> GSHMLSDEQMQIINSLVEAHHKTYDDSYSDFVRFRPPVREGPVTRSASRAASLHSLSDASSDSFNHSPESVDTKLNFSNLLMMYQDSGSPDSSEEDQQSRLSMLPHLADLVSYSIQKVIGFAKMIPGFRDLTAEDQIALLKSSAIEIIMLRSNQSFSLEDMSWSCGGPDFKYCINDVTKAGHTLEHLEPLVKFQVGLKKLKLHEEEHVLLMAICLLSPDRPGVQDHVRIEALQDRLCDVLQAYIRIQHPGGRLLYAKMIQKLADLRSLNEEHSKQY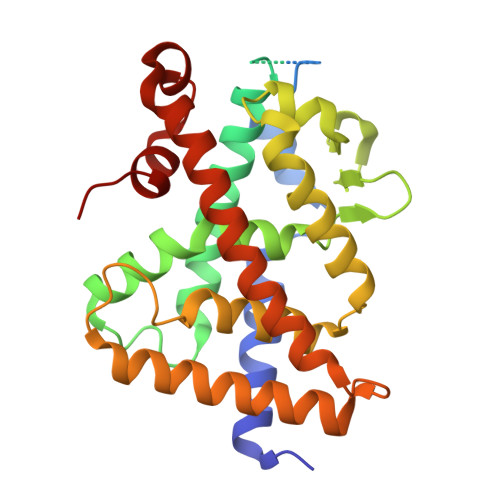RSLSFQPEHSMQLTPLVLEVFGSEVS> GSHMGGERTVTIRRQTVGGFGLSIKGGAEHNIPVVVSKISKEQRAELSGLLFIGDAILQINGINVRKCRHEEVVQVLRNAGEEV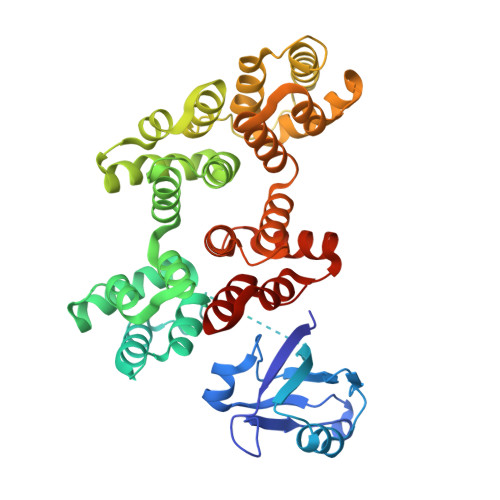TLTVSFLKRAPGSAYGSVKAYTNFDAERDALNIETAIKTKGVDEVTIVNILTNRSNEQRQDIAFAYQRRTKKELASALKSALSGHLETVILGLLKTPAQYDASELKASMKGLGTDEDSLIEIICSRTNQELQEINRVYKEMYKTDLEKDIISDTSGDFRKLMVALAKGRRAEDGSVIDYELIDQDARDLYDAGVKRKGTDVPKWISIMTERSVPHLQKVFDRYKSYSPYDMLESIRKEVKGDLENAFLNLVQCIQNKPLYFADRLYDSMKGKGTRDKVLIRIMVSRSEVDMLKIRSEFKRKYGKSLYYYIQQDTKGDYQKALLYLCGGDD>LSEEEIQRIFGLSSEQIKSLPEEXYKKXVEXTGYL[4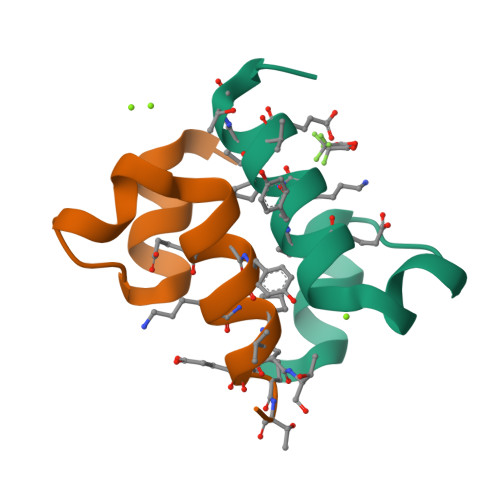x]> 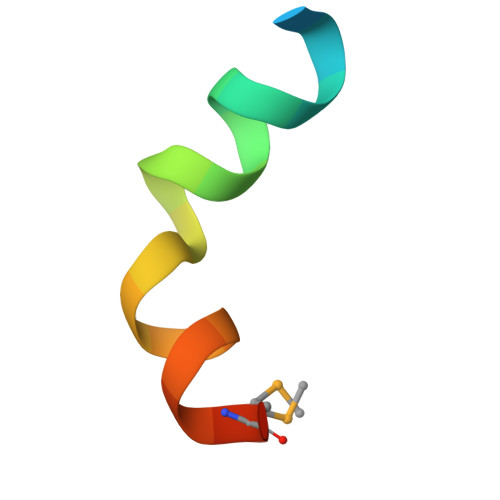ALDAEFASLFDTLDSTNKEMVNR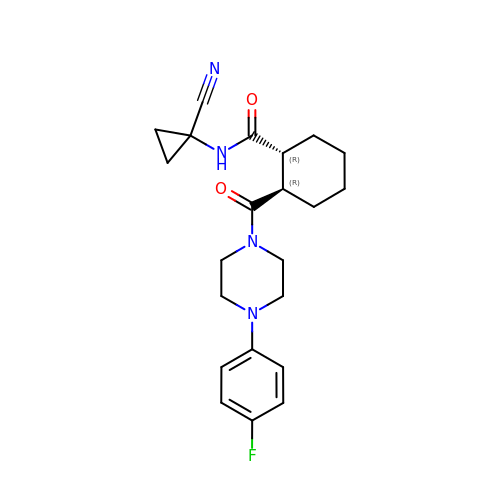(1R,2R)-N-(1-cyanocyclopropyl)-2-{[4-(4-fluorophenyl)piperazin-1-yl]carbonyl}cyclohexanecarboxamide | C22 H27 F N4 O2 | GHDIYQHGVKVLJX-RTBURBONSA-N>[2x]KGTSENKSTTA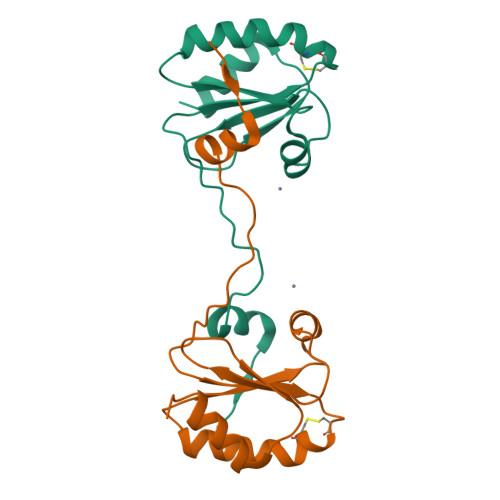TDTVQAEKPQSGTIHLTRAEFLKKIADYENHSKEWKYLGDKPAIVDFYADWCGPCKMVAPILEELSKEYAGKIYIYKVNVDKEPELARDFGIQGIPTIWFVPMKGEPQVNMGALSKEQLKGYIDKVLLKQ> MVRGFYLRFGEGVSEEANRRALALAEALLRAPPPGLLDAVPAYGVLYLEYDPRRLSRGRLLRLLKGLPQERAEEGRVVEIPVRYDGEDLPEVASRLGLSLEAVKALHQKPLYRVYALGFTPGFPFLAEVEPALRLPRKPHPRPRVPAHAVAVAGVQTGIYPLPSPGGWNLLGTSLVAVYDPHRETPFLLRPGDRVRFLEAEGP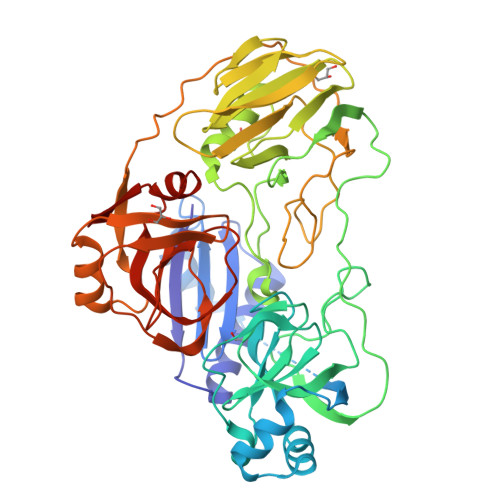TPPEPRPLELLPEEPRLPALLVEEPGLMDLVVDGGRFLGGHLGLARSGPLDAPSARLANRLVGNGAGAPLLEFAYKGPVLTALRDLVAAFAGYGFVALLEGEEIPPGQSFLWPRGKTLRFRPRGPGVRGYLAVAGGLEVRPFLGSASPDLRGRIGRPLWAGDVLGLEALRPVRPGRAFPQRPLPEAFRLRLLPGPQFAGEAFRALCSGPFRVARADRVGVELLGPEVPGGEGLSEPTPLGGVQVPPSGRPLVLLADKGSLGGYAKPALVDPRDLWLLGQARPGVEIHFTSG>[2x]GAVFEFDNLAPMLATHGTVAGLKASQWAFEGKWDGYRLLVEADHGAVRLRSRSGRDVTAEYPQLRALAEDLADHHVVLDGEAVVLDSSGVPSFSQMQNRGRDTRVE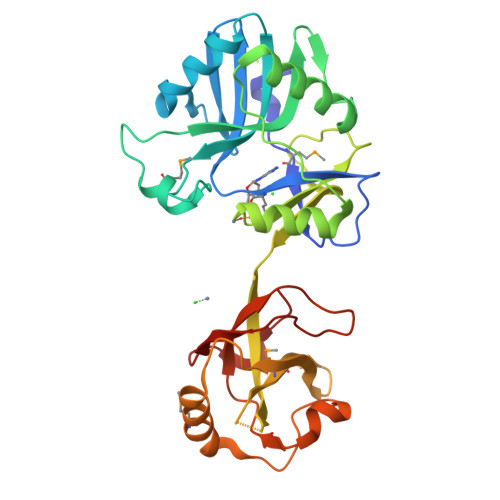FWAFDLLYLDGRALLGTRYQDRRKLLETLANATSLTVPELLPGDGAQAFACSRKHGWEGVIAKRRDSRYQPGRRCASWVKDKHWNTQEVVIGGWRAGEGGRSSGVGSLLMGIPGPGGLQFAGRVGTGLSERELANLKEMLAPLHTDESPFDVPLPARDAKGITYVKPALVAEVRYSEWTPEGRLRQSSWRGLRPDKKPSEVVRE>[2x]SNAMT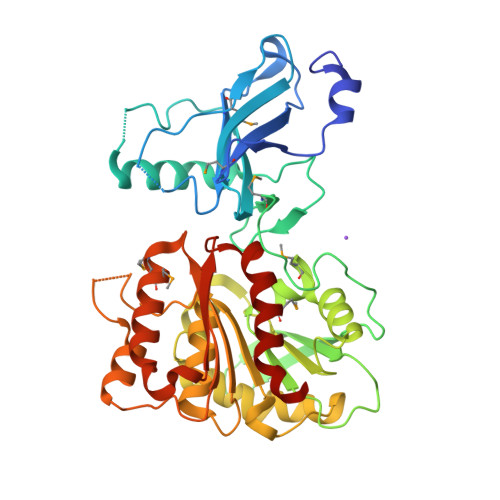ALKVGSESWWQSKHGPEWQRLNDEMFEVTFWWRDPQGSEEYSTIKRVWVYITGVTDHHQNSQPQSMQRIAGTDVWQWTTQLNANWRGSYCFIPTERDDIFSAPSPDRLELREGWRKLLPQAIADPLNPQSWKGGLGHAVSALEMPQAPLQPGWDCPQAPEIPAKEIIWKSERLKNSRRVWIFTTGDVTAEERPLAVLLDGEFWAQSMPVWPVLTSLTHRQQLPPAVYVLIDAIDTTHRAHELPCNADFWLAVQQELLPLVKVIAPFSDRADRTVVAGQSFGGLSALYAGLHWPERFGCVLSQSGSYWWPHRGGQQEGVLLEKLKAGEVSAEGLRIVLEAGIREPMIMRANQALYAQLHPIKESIFWRQVDGGHDALCWRGGLMQGLIDLWQPLFHDRS>MRGSHHHHHTTGEDDESECVINYVEKAVNKLTLQMPYQLFIGGEFVDAEGSKTYNTINPTDGSVICQVSLAQVSDVDKAVAAAKEAFENGLWGKINARDRGRLLYRLADVMEQHQEELATIEALDAGAVYTLALKTHVGMSIQTFRYFAGWCDKIQGATIPINQARPNRNLTLTKKEPVGVCGIVIPWNYPLMMLSWKTAACLAAGNTVVIKPAQVTPLTALKFAELTLKAGIPKGVVNILPGSGSLVGQRLSDHPDVRKIGFTGSTEVGKHIMKSCALSNVKKVSLALGGKSPLIIFADCDLNKAVQMGMSSVFFNKGENAIAAGRLFVEESIHNQFVQKVVEEVEKMKIGNPLERDTNHGPQNHEAHLRKLVEYCQRGVKEGATLVCGGNQVPRPGFFFQPTVFTDVEDHMYIAKEESFGPIMIISRFADGDVDAVLSRANATEFGLASGVFTRDINKALYVSDKLQAGTVFINTYNKTDVAAPFGGFKQSGFGKDLGEAALNEYLRIKTVTFEY[4x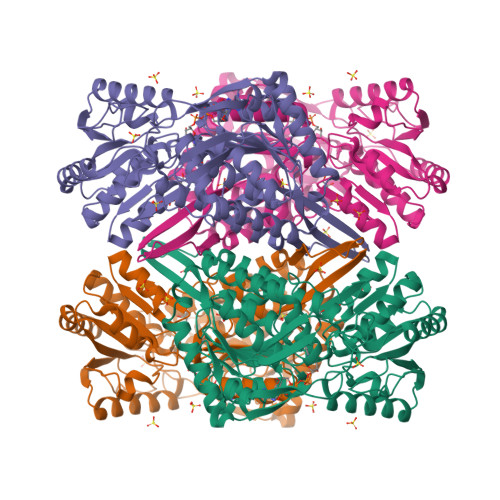]>[2x]LPNITILATGGTIAGGGDSATKSNYTVGKVGVENLVNAVPQLKDIANVKGEQVVNIGSQDMNDNVWLTLAKKINTDCDKTDGFVITHGTETMEETAYFLDLTVKCDKPVVMVGAMRPSTSMSADGPFNLYNAVVTAADKASANRGVLVVMNDTVLDGRDVTKTNTTDVATFKSVNYGPLGYIHNGKIDYQRTPARKHT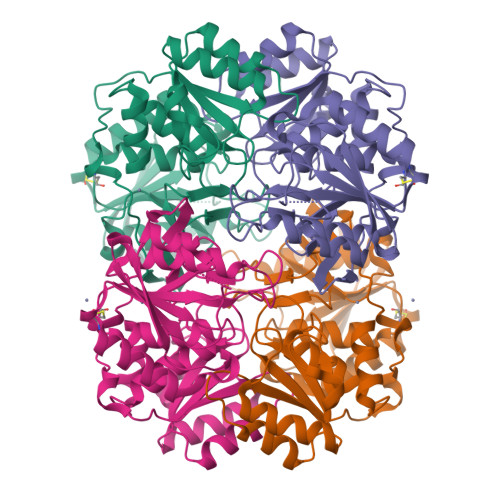SDTPFDVSKLNELPKVGIVYNYANASDLPAKALVDAGYDGIVSAGVGNGNLYKSVFDTLATAAKTGTAVVRSSRVPTGATTQDAEVDDAKYGFVASGTLNPQKARVLLQLALTQTKDPQQIQQIFNQY(2E,5R)-5-(2-cyclohexylethyl)-5-{[(3R)-1-(cyclopentylacetyl)pyrrolidin-3-yl]methyl}-2-imino-3-methylimidazolidin-4-one 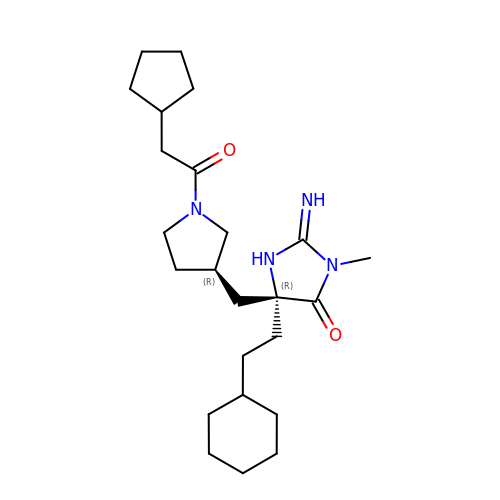| C24 H40 N4 O2 | ZROUWOKUKKGJPH-HYBUGGRVSA-N6-[(3~{a}~{S},4~{S},6~{a}~{R})-2-oxidanylidene-1,3,3~{a},4,6,6~{a}-hexahydrothieno[3,4-d]imidazol-4-yl]-~{N}-(2,2,6,6-tetramethyl-1-oxidanyl-piperidin-4-yl)hexanamide | C20 H36 N4 O3 S | 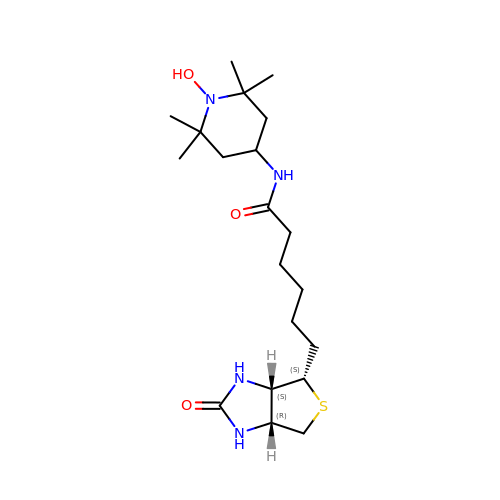PUXBASNOQZMIKI-ZOBUZTSGSA-N> SDELYRQSLEIISRYLREQATGAKDTKPMGRSGATSRKALETLRRVGDGVQRNH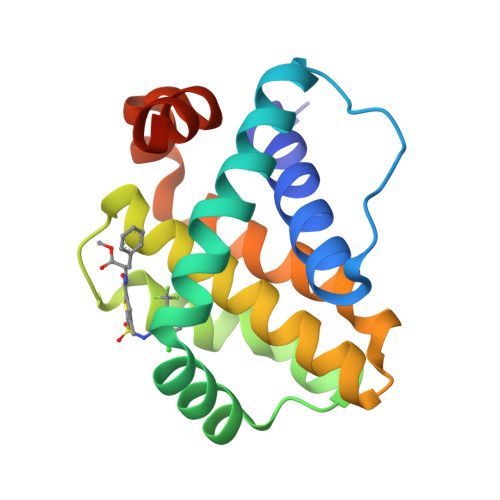ETAFQGMLRKLDIKNEDDVKSLSRVMIHVFSDGVTNWGRIVTLISFGAFVAKHLKTINQESCIEPLAESITDVLVRTKRDWLVKQRGWDGFVEFFHVEDLEGG> AEQISHKKSLRVSSLNKDRRLLLREFYNL;> MNNSEDPFQQVVKDTKEQLNRINNYITRHNTAGDDDQEEEIQDILKDVEETIVDLDRSIIVMKR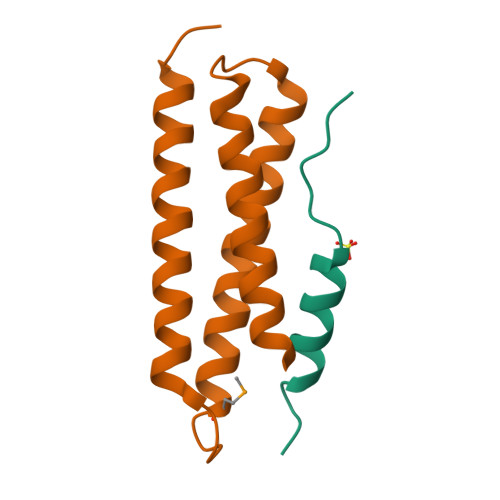DENEDVSGREAQVKNIKQQLDALKLRFDRRIQESTQT> MIDVAIAIDAESVEVTWRNRSGGSYDSRGNATGASWADTQIRAAI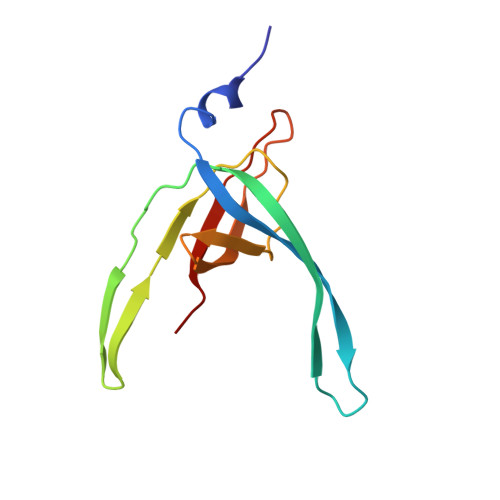QPVSGRELQDLPEGVRSKVTLVAWTRSEVAENDQIIYLGDAYRVYAARPRPMDGFTRIALGKVSP> GLTYSQTMELKDSMLQLDPNAKTWIDIEGRPEDPVEIAIYQPNNGQYIHFYREPTDIKQFKQDSKHSHGIDIQDLFSVQPGLTSA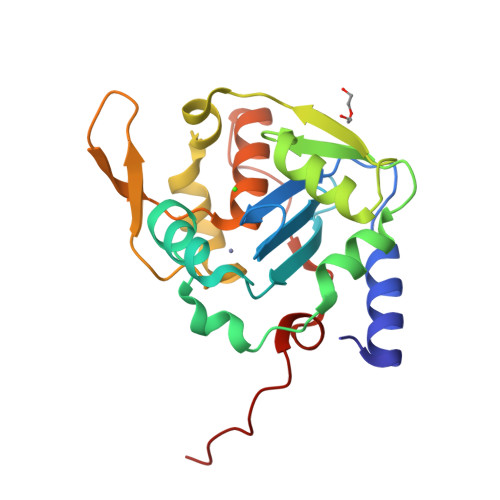VIESLPKNMVLSCQGADDIRKLLDSQNRRDIKLIDVSMQKDDARKFEDKIWDEYKHLCRMHTGIVTQKKKRGGKEEVTPHCALLDCLMFEAAVIGSPQIPTPRPVLSRDLVFRTGPPRVVL> MKTAILAAMLGSAAAFVPAQQSKVSTSLAASELEDGIGAVAPLGYFDPLGYIKDEETFIRYRAVERKHGRVAMMAMLGTFVHNNGWTFDGYLSPSQGLKFSDIDSGIGGLFQVPPAGLAQIILLCGFVELAWWPASNLSGDY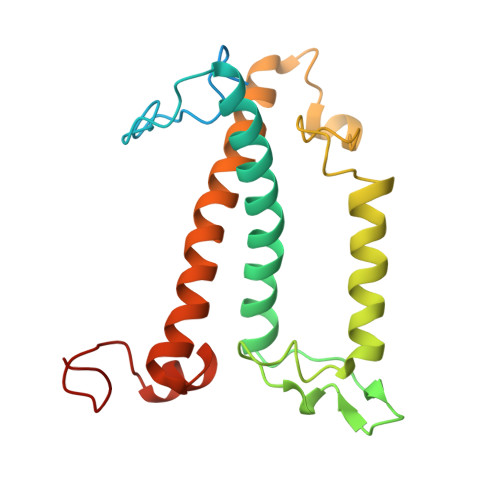GVRLGTLNDWEEQPAKYYRQKNAELNNGRAAMMGILGTFTHEVITGQNFAEQAAAGHFSPFGDGQGFF>[3x]MFEARLVQGSILKKVLEALKDLINEACWDISSSGVNLQSMDSSHVSLVQLTLRSEGFDTYRCDRNLAMGVNLTSMSKILKCAGNEDIITLRAEDNADTLALVFEAPNQEKVSDYEMKLMDLDVEQLGIPEQE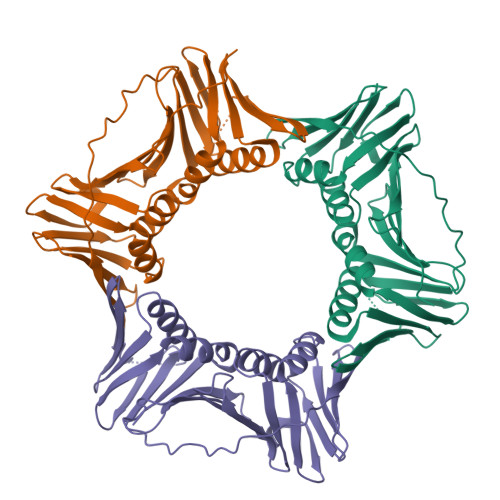YSCVVKMPSGEFARICRDLSHIGDAVVISCAKDGVKFSASGELGNGNIKLSQTSNVDKEEEAVTIEMNEPVQLTFALRYLNFFTKATPLSSTVTLIMSADVPLVVEYKIADMGHLKYYLAPKIEDEEGS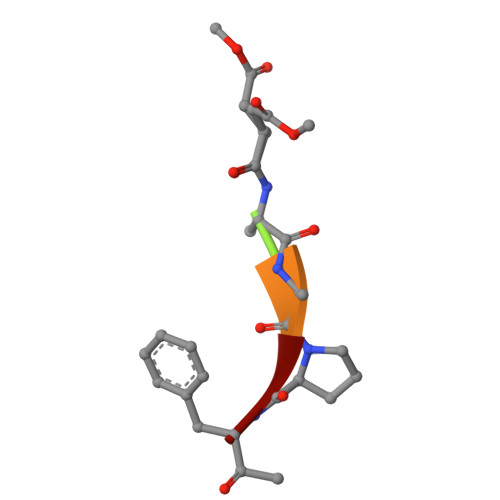> XAAPF>[2x]MRGSHHHHHHGSMKQLTILGSTGSIGCSTLDVVRHNPEHFRVVALVAGKNVTRMVEQCLEFSPRYAVMDDEASAKLLKTMLQQQGSRTEVLSGQQAACDMAALEDVDQVMAAIVGAAGLLPTLAAIRAGKTILLANKESLVTCGRLFMDAVKQSKAQLLPVDSEHNAIFQSLPQPIQHNLGYADLEQNGVVSILLTGSGGPFRETPLRDLATMTPD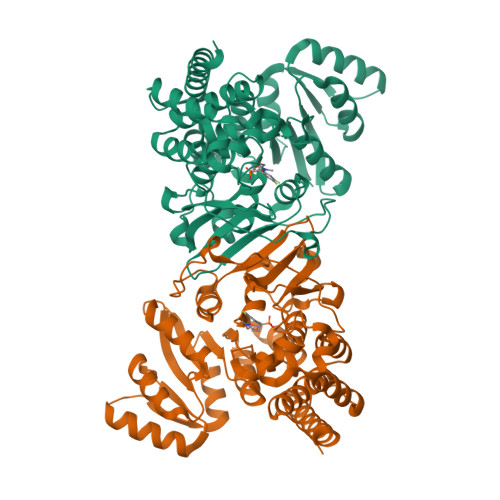QACRHPNWSMGRKISVDSATMMNKGLEYIEARWLFNASASQMEVLIHPQSVIHSMVRYQDGSVLAQLGEPDMRTPIAHTMAWPNRVNSGVKPLDFCKLSALTFAAPDYDRYPCLKLAMEAFEQGQAATTALNAANEITVAAFLAQQIRFTDIAALNLSVLEKMDMREPQCVDDVLSVDANAREVARKEVMRLAS4-amino-3-fluoro-N-(1-{[(2Z)-2-iminoethyl]carbamoyl}cyclohexyl)benzamide 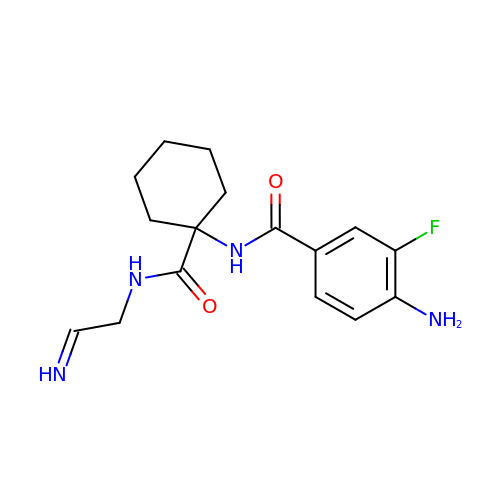| C16 H21 F N4 O2 | ULJOBOHEOALILQ-LSCVHKIXSA-N>MPEAWIVEAVRTPIGKHGGALASVRPDDLLAHALSVLVDRSGVPKEEVEDVYAGCANQAGEDNRNVARMALLLAGFPVEVAGCTVNRLCGSGLEAVAQAARAIWAGEGKVYIGSGVESMSRAPYAVPKPERGFPTGNLVMYDTTLGWRFVNPKMQALYGTESMGETAENLAEMYGIRREEQDRFALLSHQKAVRAWEEGRFQDEVVPVPVKRGKEEILVEQDEGPRRDTSLEKLAALRPVFREGGTVTAGNSSPLNDGAAAVLLVSDDYAKAHGLRPLARVRAIAVAGVPPRIMGIGPVPATRKALERAGLSFSDL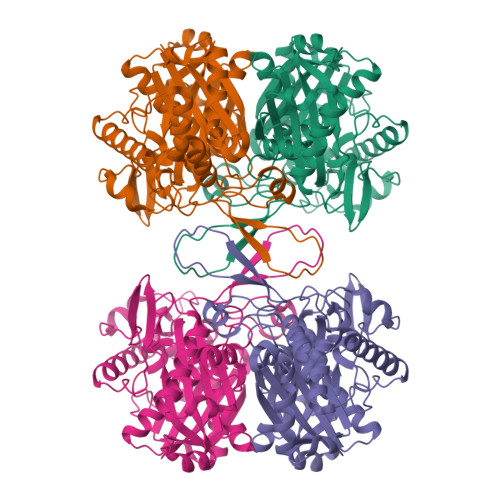GLIELNEAFAAQALAVLREWSLSMEDQRLNPNGGAIALGHPLGASGARILTTLVHEMRRRKVQFGLATMCIGVGQGIAVVVEGMG[8x]> MSLSWEIEELDREIGKIKKHSLILIHEEDASSRGKDILFYILSRKLKSDNLVGMFSISYPLQLIIRI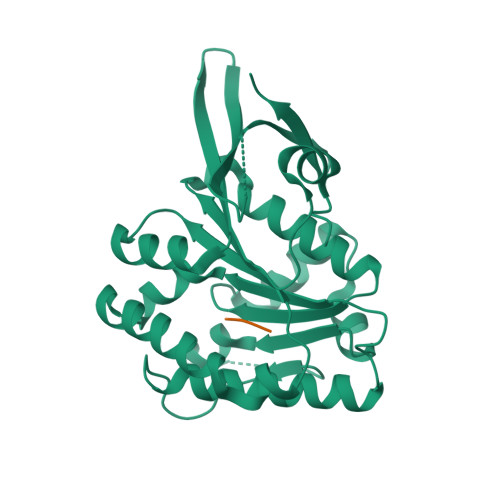LSRFGVDVIKYLENHRLAIVDTFGSFHGIKATMPGVWYLEGMLSSETLPIKYAKAVEDHKKVWMDLNLFEGRELYGFAISMSGYLEVFTPEETLRYLETSAEVRYGHPAYKKYPRGTNFWLWEGVKDKRVLLSVYRRADYVLKTRSSLGENGIKRELLVIKTPKPIEELVRFEYEFKGNEPKLRREGHHHHHH;> NIF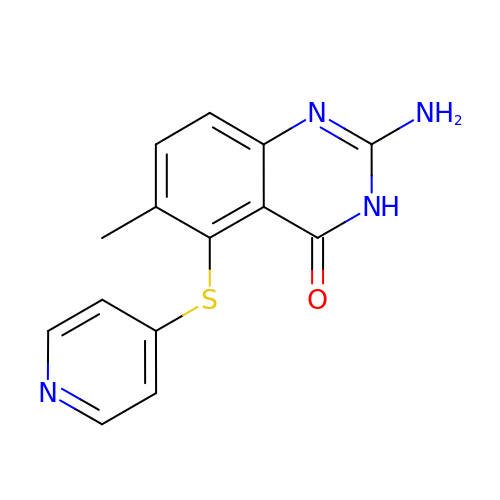2-azanyl-6-methyl-5-pyridin-4-ylsulfanyl-3H-quinazolin-4-one | C14 H12 N4 O S | XHWRWCSCBDLOLM-UHFFFAOYSA-N methyl 4-(2,3-dihydroindol-1-yl)-4-oxidanylidene-butanoate | 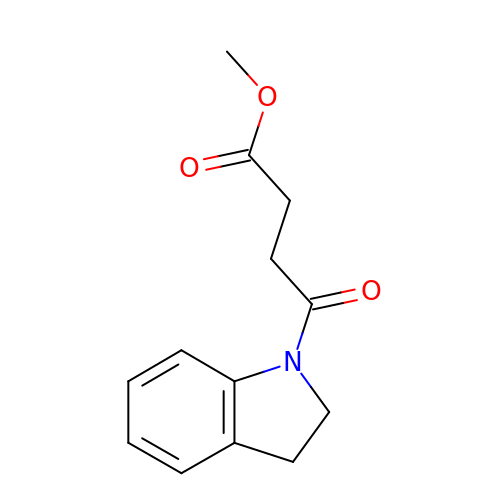C13 H15 N O3 | AYMVNVWATJUROX-UHFFFAOYSA-N> MVFQSHIGVLAFPFGTHAAPLLTVVQRLATSSPHTLFSFFNSAVSNSTLFNNGVLDSYDNIRVYHVWDGTPQGQAFTGSHFEAVGLFLKASPGNFDKVIDEAEVETGLKISCLITDAFLWFGYDLAEKRGVPWLAFWTSAQCALSAHMYTHEILKAVGSNGVGETAEEELIQSLIPGLEMAHLSDLPPEIFFDKNPNPLAITINKMVLKLPKSTAVILNSFEEIDPIITTDLKSKFHHFLNIGPSILSSPTPPPPDDKTGCLAWLDSQTRPKSVVYISFGTVITPPENELAALSEALETCNYPFLWSLNDRAKKSLPTGFLDRTKELGMIVPWAPQPRVLAHRSVGVFVTHCGWNSILESICSGVPLICRPFFGSDHKLNSRMVEDSWKIGVRLEGGVLSKTATVEALGRVMMSEEGEIIRENV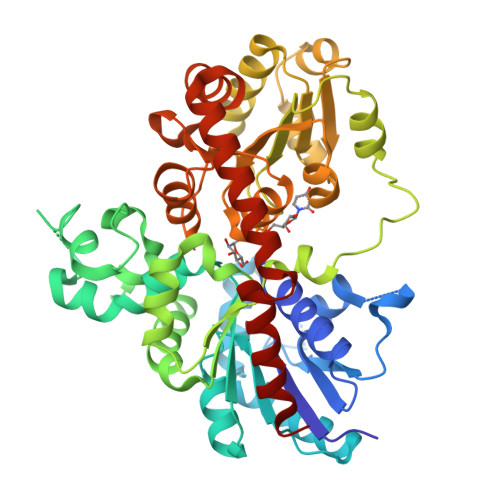NEMNEKAKIAVEPKGSSFKNFNKLLEIINAPQSS> MSQGTFTSDYSKYLDSRRAQDFVQW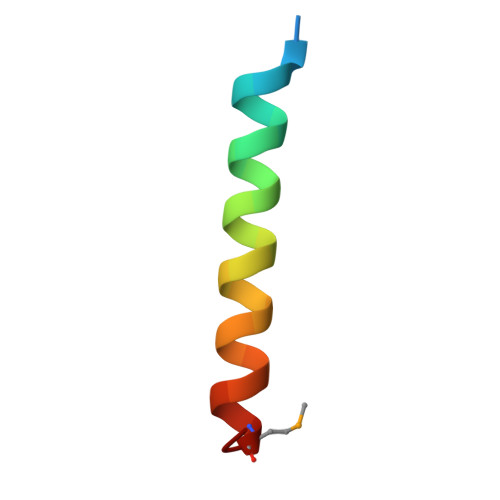LMNT> MANSTAELEELLMQRSLTDPQLQAAAAAAADFRILPDATVIKIGGQSVIDRGRAAVYPLVDEIVAARKNHKLLIGTGAGTRARHLYSIAAGLGLPAGVLAQLGSSVADQNAAMLGQL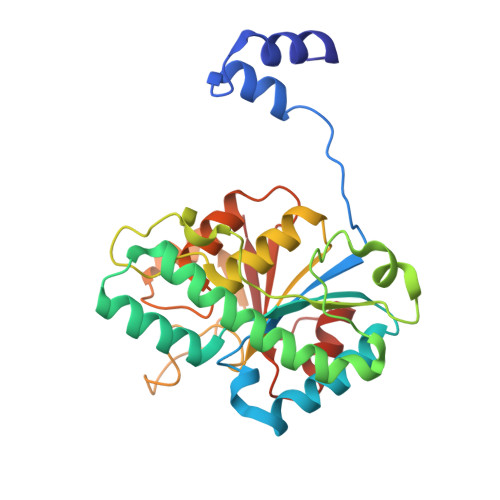LAKHGIPVVGGAGLSAVPLSLAEVNAVVFSGMPPYKLWMRPAAEGVIPPYRTDAGCFLLAEQFGCKQMIFVKDEDGLYTANPKTSKDATFIPRISVDEMKAKGLHDSILEFPVLDLLQSAQHVREVQVVNGLVPGNLTRALAGEHVGTIITAS> MDSTNLNKRPLLQYSLSSLGSQITKWSSSRPTSPVRKARSTENDFLSKQDTSSILPSINDDGGEQWYEKFKPNCLEQVAIHKRKLKDVQEALDAMFLPNAKHRILLLSGPSGCSKSTVIKELSKILVPKYRQNSNGTSFRSTPNEHKVTEFRGDCIVNDLPQMESFSEFLKGARYLVMSNLSLILIEDLPNVFHIDTRRRFQQLILQWLYSSEPLLPPLVICITECEIPENDNNYRKFGIDYTFSAETIMNKEILMHPRLKRIKFNPINSTLLKKHLKFICVQNMKMLKEKNKWNKRQEVIDYIAQETGDIRSAITTLQFWATSSGSLPISTRESTISYFHAIGKVIHGSHSTNNDNEMINNLFENSNNLLSKEDFKLGILENYNTFNKGEFSISDASSIVDCLSECDNMNGLPESNEYGLREVRKTFRNISKQGHNHGTVYFPREWKVRKLQNSFKVQAEDWLNVSLYKYNAVHSFRNITLEFGYYAPLIRKCQSYKKKYILYYLKNLPSGSSGPKQTMDKFSDIMKVENGIDVVDRIGGPIEALSVEDGLAPLMDNDSNNCDHLEDQKKERDRRLRMLIDQYERNVMMANDDLEDEETSFNDDPIVDSDSDNSNNIGNETFGRSDEDESLCEILSQRQPRKAPVISESLSDSDLEIL;> MSKTLSLQLPWVEKYRPQVLSDIVGNKETIDRLQQIAKDGNMPHMIISGMPGIGKTTSVHCLAHELLGRSYADGVLELNASDDRGIDVVRNQIKHFAQKKLHLPPGKHKIVILDEADSMTAGAQQALRRTMELYSNSTRFAFACNQSNKIIEPLQSRCAILRYSKLSDEDVLKRLLQIIKLEDVKYTNDGLEAIIFTAEGDMRQAINNLQSTVAGHGLVNADNVFKIVDSPHPLIVKKMLLASNLEDSIQILRTDLWKKGYSSIDIVTTSFRVTKNLAQVKESVRLEMIKEIGLTHMRILEGVGTYLQLASMLAKIHKLNNKA;> MSTSTEKRSKENLPWVEKYRPETLDEVYGQNEVITTVRKFVDEGKLPHLLFYGPPGTGKTSTIVALAREIYGKNYSNMVLELNASDDRGIDVVRNQIKDFASTRQIFSKGFKLIILDEADAMTNAAQNALRRVIERYTKNTRFCVLANYAHKLTPALLSRCTRFRFQPLPQEAIERRIANVLVHEKLKLSPNAEKALIELSNGDMRRVLNVLQSCKATLDNPDEDEISDDVIYECCGAPRPSDLKAVLKSILEDDWGTAHYTLNKVRSAKGLALIDLIEGIVKILEDYELQNEETRVHLLTKLADIEYSISKGGNDQIQGSAVIGAIKASFENETVKANV;> MFEGFGPNKKRKISKLAAEQSLAQQPWVEKYRPKNLDEVTAQDHAVTVLKKTLKSANLPHMLFYGPPGTGKTSTILALTKELYGPDLMKSRILELNASDERGISIVREKVKNFARLTVSKPSKHDLENYPCPPYKIIILDEADSMTADAQSALRRTMETYSGVTRFCLICNYVTRIIDPLASRCSKFRFKALDASNAIDRLRFISEQENVKCDDGVLERILDISAGDLRRGITLLQSASKGAQYLGDGKNITSTQVEELAGVVPHDILIEIVEKVKSGDFDEIKKYVNTFMKSGWSAASVVNQLHEYYITNDNFDTNFKNQISWLLFTTDSRLNNGTNEHIQLLNLLVKISQL;> MSLWVDKYRPKSLNALSHNEELTNFLKSLSDQPRDLPHLLLYGPNGTGKKTRCMALLESIFGPGVYRLKIDVRQFVTASNRKLELNVVSSPYHLEITPSDMGNNDRIVIQELLKEVAQMEQVDFQDSKDGLAHRYKCVIINEANSLTKDAQAALRRTMEKYSKNIRLIMVCDSMSPIIAPIKSRCLLIRCPAPSDSEISTILSDVVTNERIQLETKDILKRIAQASNGNLRVSLLMLESMALNNELALKSSSPIIKPDWIIVIHKLTRKIVKERSVNSLIECRAVLYDLLAHCIPANIILKELTFSLLDVETLNTTNKSSIIEYSSVFDERLSLGNKAIFHLEGFIAKVMCCLD;> MKLKLIVNGCEAPDDYKLLRTTINTVASLRKTAILRFNSERLTIISTPKSSLNSSNNGTILRGDT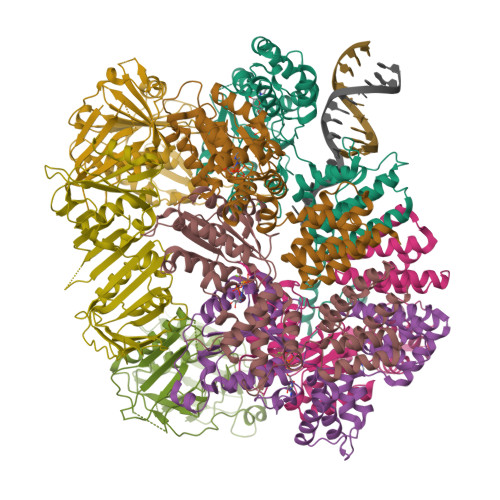GQLWCTIPHDVFRLYTVISARELNTITMECNCDSLLSVFKRYDRVMNQGSSSNMTIKLQSCALGITFEEIVHTSGPNDAIVMNGGVDEHNGLPTTVGTGNLLASNKVIMHSFKVPVKLLFRAQDTRIQEPMINYIQLMMYKLPPISGEFGSAFHGFIRRVERYSNVNHIHLMGVKKKEHGNEGDDVELKIIVNELDWHLEICWNGPLDSVIQRQEGLTDNPSQNQHIDTDGRQEEGSLPIIEADKPMSSLYTNTRDREMEENIRYDEDLLRIEDSSIADTRGNIYTADTSGDTEFNDISVMVEKAEQESSSTHEVIIRCKDWKVCSKLYAAFEEVVLAISHDESCVFHCSLDRGSLEDSEDVEKPRERGQIIYYIARSKGL;> MRINSELANKFSASTVHLEHITTALSCLTPFGSKDDVLIFIDADGLSFVRENNHVIKIQLLLSRELFMSYSYRNETEDHMKLCVKINHILDSVSVMNRNSDDIVECTLSYDGHGSPFVLIFEDSFISERVEYSTYLIKDFDTNGLELDRERISFEAIIKGEALHSALKDLKEIGCKECYVYAKTEANDENVFALISKSQLGFSKIKLPSNRSILEKLQVFDGDSTTVIDGFAVIGFFDFTSFDKIRKSTKIASKVLFRMDVHGVLSVNILSQTDDVIITDTTRPSNNRPGSIRQLQLPKDYPGIVIEVCMLEKESIDEAAQTEIELLMETNELGNRNSFKKSTIRKRYGTDKGNETSNDNLLQLNGKKIKLPSEEENNKNRESEDEENHCKYPTKDIPIFF;> MSFKATITESGKQNIWFRAIYVLSTIQDDIKITVTTNELIAWSMNETDTTLCQVRFQKSFFEEYEFKPHEIVFGENGVQVIEDTYGNSHKLYSFRVNGRHLTTISRKPDGDGIKSFTIAVNNTSTCPESLANRLIVVIEMDSLIVKEYCPQFQPIKYDPIIINLKYKRRFLDVFGTAASDRNPQEPLDPKLLDVFTNTERELTSALFNEEVESDIRKRNQLTAADEINYICCNSTLLKNFLDNCNVNVTDEVKLEINVHRLSITAFTKAVYGKNNDLLRNALSMSNTISTLDLEHYCLFTTIEDEKQDKRSHSKRREHMKSIIFKLKDFKNFITIGPSWKTTQDGNDNISLWFCHPGDPILMQMQKPGVKLELVEVTDSNINDDILEGKFIKTAISGSKEEAGLKDNKESCESPLKSKTALKRENLPHSVAGTRNSPLKVSYLTPDNGSTVAKTYRNNTARKLFVEEQSQSTNYEQDKRFRQASSVHMNMNREQSFDIGTTHEVACPRNESNSLKRSIADICNETEDPTQQSTFAKRADTTVTWGKALPAADDEVSCSNIDRKGMLKKEKLKHMQGLLNSQNDTSNHKKQDNKEMEDGLGLTQVEKPRGIFD>MSPIVSVPDITAPVENVPAILPKVVPGELIVNKPTGGDSDELFQYLVDILASPVYDVAIESPLELAEKLSDRLGVNFYIKREDKQRVFSFKLRGAYNMMSNLSREELDKGVITASAGNHAQGVALAGQRLNCVAKIVMPTTTPQIKIDAVRALGGDVVLYGKTFDEAQTHALELSEKDGLKYIPPFDDPGVIKGQGTIGTEINRQLKDIHAVFIPVGGGGLIAGVATFFKQIAPNTKIIGVEPYGAASMTLSLHEGHRVKLSNVDTFADGVAVALVGEYTFAKCQELIDGMVLVA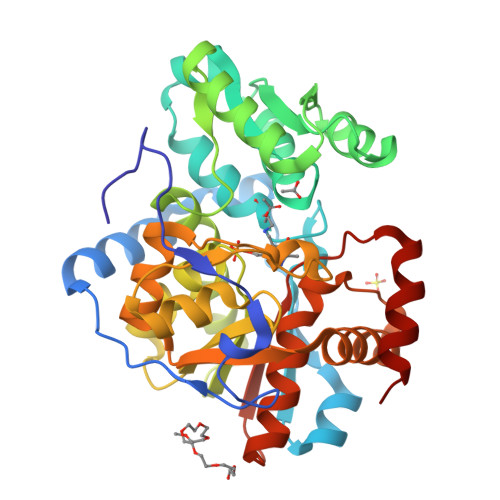NDGISAAIKDVYDEGRNILETSGAVAIAGAAAYCEFYKIKNENIVAIASGANMDFSKLHKVTELAGLGSGK[2x]>SYTLPSLPYAYDALEPHFDKQTMEIHHTKHHQTYVNNANAALESLPEFANLPVEELITKLDQLPADKKTVLRNNAGGHANHSLFWKGLKKGTTLQGDLKAAIERDFGSVDNFKAEFEKAAASRFGSGWAWLVLKGDKLAVVSTANQDSPLMGEAISGASGFPIMGLDVWEHA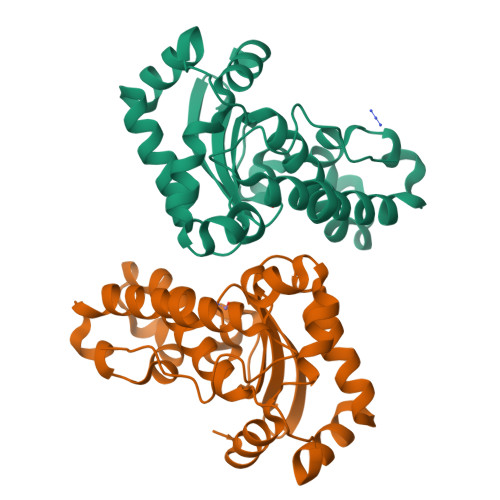YFLKFQNRRPDYIKEFWNVVNWDEAAARFAAKK[2x]>DNILYSGETLSPGEFLNNGRYVFIMQEDCNLVLYDVDKPIWATNTGGLDRRCHLSMQSDGNLVVYSPRNNPIWASNTGGENGNYVCVLQKDRNVVIYGTARWATGTNIH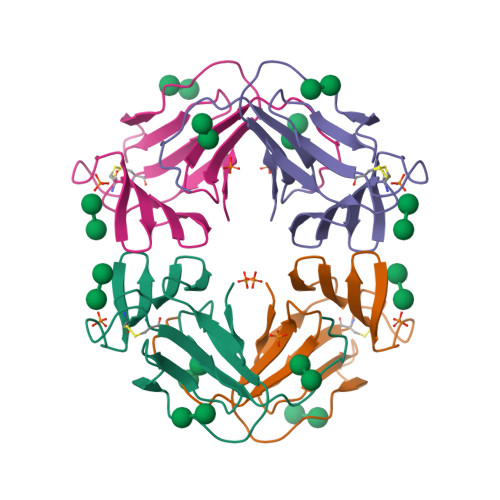[2x]> MDLLAELQWRGLVNQTTDEDGLRKLLNEERVTLYCGFDPTADSLHIGHLAAILTMRRFQQAGHRPIALVGGATGLIGDPSGKKSERTLNAKETVEAWSARIKEQLGRFLDFEA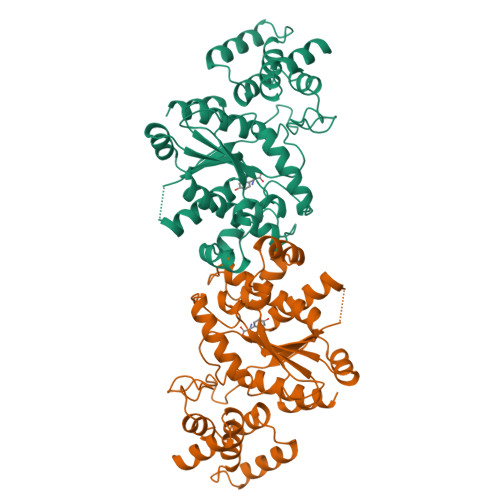DGNPAKIKNNYDWIGPLDVITFLRDVGKHFSVNYMMAKESVQSRIETGISFTEFSYMMLQAYDFLRLYETEGCRLQIGGSDQWGNITAGLELIRKTKGEARAFGLTIPLVTKADGTKFGKTESGTIWLDKEKTSPYEFYQFWINTDDRDVIRYLKYFTFLSKEEIEALEQELREAPEKRAAQKTLAEEVTKLVHGEEALRQAIRIS>MKTLIEIKQTPDGIIKADKVFNKVKDKISLPNRILYLGCGSSHFLSKLLAMVTNMHGGLGIALPCSEFLYSKETYPIGEVELAVGISRSGETTEILLALEKINVKKLGITTRESSLTRMCDYSLVVPAIEESVVMTHSFTSFYFAYLQLLRYSYGLPPLNAGEISKATEKSLEYERYIREIVESFDFQNIIFLGSGLLYPVALEASLKMKEMSIFWSEAYPTFEVRHGFKAIADEKTLVVLMVEEPFEWHEKLVKEFKNQGAKVLVISNSPQDLGQDYSIELPRLSKDANPIPYLPIVQLLSYY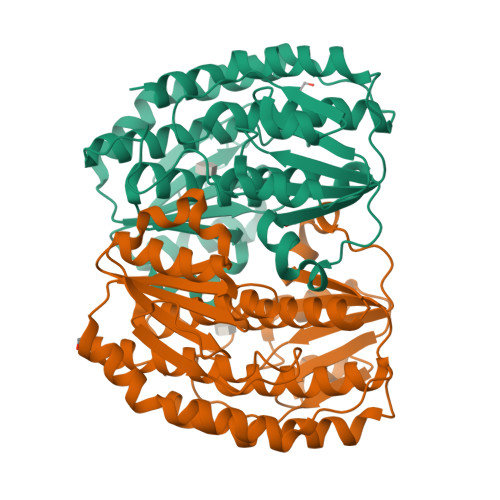KAVSRGLNPDNPRFLDKVVRW[2x]>MGWSHPQFEKENLYFQGSATEKYYIRDAITKPAVHHESYQKLWETKWKKPCEMGVYPFMFGSIKDFEPVAQEIIKKGLKEPYDWDEYAQMYFPKAEELAKIAEEAEAAGEKEKASEYYLRSSAVYRISRFPTPRSEKQKYAWRKGCEVFYKGAALMEYPIKEVRIPHKHGIEGEGDVVPVNFLLPPNASETSPVPCVLIITGLDGYRTELAVWQQGWRSKGVATVIAEIPGTGDSPALRQDPTSPDRQWSSVLDWIESQKAVDSKKIVAWGFSTGGYYALRMAHTHKDRLLATISLGGGAHHMFDREWLEHANKLEYPFDLSNTLAYKFGYPDLESFIEESSKFSLLNDGTLQKPCTKVLLVNGNDDEIFPIDDMFVSLENGQPKLARM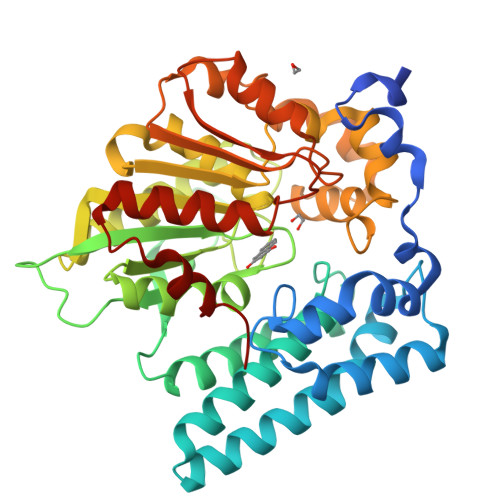VKGKKHMGEPESFSIILEWIHKLLGLDGKIKEQLAMIPSRTK[2x]>[3x]MRCIGISNRDFVEGVSGGSWVDIVLEHGSCVTTMAKNKPTLDFELIKTEAKQPATLRKYCIEAKLTNTTTDSRCPTQGEPTLNEEQDKRFVCKHSMVDRGWGNGCGLFGKGGIVTCAMFTCKKNMEGKIVQPENLEYTVVITPHSGEEHAVGNDTGKHGKEVKITPQSSITEAELTGYGTVTMECSPRTGLDFNEMVLLQMKDKAWLVHRQWFLDLPLPWLPGADTQGSNWI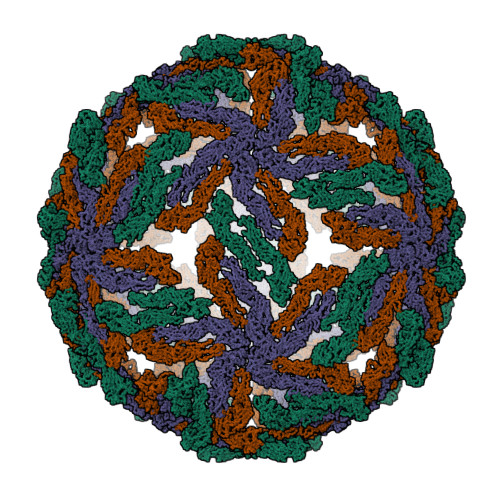QKETLVTFKNPHAKKQDVVVLGSQEGAMHTALTGATEIQMSSGNLLFTGHLKCRLRMDKLQLKGMSYSMCTGKFKVVKEIAETQHGTIVIRVQYEGDGSPCKIPFEIMDLEKRHVLGRLITVNPIVTEKDSPVNIEAEPPFGDSYIIIGVEPGQLKLDWFKKGSSIGQMFETTMRGAKRMAILGDTAWDFGSLGGVFTSIGKALHQVFGAIYGAAFSGVSWTMKILIGVIITWIGMNSRSTSLSVSLVLVGIVTLYLGVMVQA>[2x]GKAVIAIHGGAGAISRAQMSLQQELRYIEALSAIVETGQKMLEAGESALDVVTEAVRLLEECPLFNAGIGAVFTRDETHELDACVMD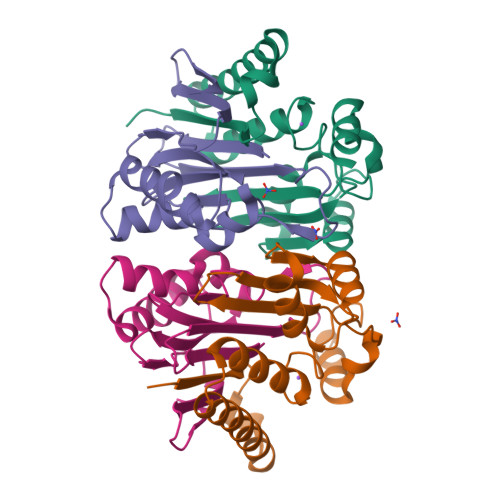GNTLKAGAVAGVSHLRNPVLAARLVMEQSPHVMMIGEGAENFAFARGMERVSPEIFSTSLRYEQLLAARKEGATVLDHSGAPLDEKQKMG;>TVGAVALDLDGNLAAATSTGGMTNKLPGRVGDSPLVGAGCYANNASVAVSCTGTGEVFIRALAAYDIAALMDYGGLSLAEACERVVMEKLPALGGSGGLIAIDHEGNVALPFNTEGMYRAWGYAGDTPTTGIYREKGDTVATQHSIE[2x]(1S)-1-[(3R,5R,7R)-tricyclo[3.3.1.1~3,7~]decan-1-yl]ethan-1-amine | C12 H21 N | 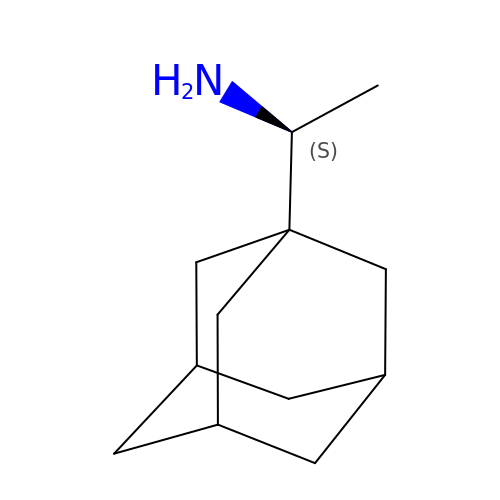UBCHPRBFMUDMNC-SVNGYHJRSA-N>GIDPFTMAAYTIVKEEESPIAPHRLFKALVLERHQVLVKAQPHVFKSGEIIEGDGGVGTVTKITFVDGHPLTYMLHKFDEIDAANFYCKYTLFEGDVLRDNIEKVVYEVKLEAVGGGSKGK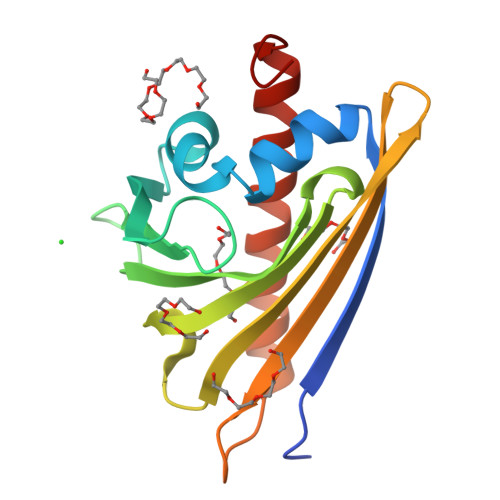ITVTYHPKPGCTVNEEEVKIGEKKAYEFYKQVEEYLAANPEVFA[2x]> KSYIDRDTEYLLQENEPNLSLDQHLLEDLQRKKTDPRYIEMQRFRKKLPSYGMQKELVNLINNHQVTVISGETGCGKTTQVTQFILDNYIERGKGSACRIVCTQPRRISAISVAERVATERAESCGNGNSTGYQIRLQSRLPRKQGSILYCTTGIILQWLQSDSRLSSVSHIVLDEIHERNLQSDVLMTVIKDLLHFRSDLKVILMSATLNAEKFSEYFGNCPMIHIPGFTFPVVEYLLEDIIEKIRYVPDQKEHRSQFKRGFMQGHVNRQEKEEKEAIYKERWPAYIKELRTRYSASTVDVLQMMDDDKVDLNLIAALIRYIVLEEEDGAILVFLPGWDNISTLHDLLMSQVMFKSDKFLIIPLHSLMPTVNQTQVFKKTPPGVRKIVIATNIAETSITIDDVVYVIDGGKIKETHFDTQNNISTMSAEWVSKANAKQRKGRAGRVQPGHCYHLYNGLRASLLDDYQLPEILRTPLEELCLQIKILRLGGIAYFLSRLMDPPSNEAVVLSIKHLMELSALDKQEELTPLGVHLARLPVEPHIGKMILFGALFCCLDPVLTIAASLSFKDPFVIPLGKEKIADARRKELAKETRSDHLTVVNAFEGWEEAKRRGFRYEKDYCWEYFLSSNTLQMLHNMKGQFAEHLLGA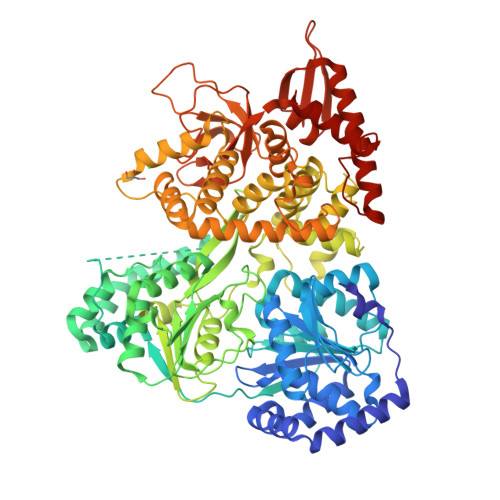GFVSSRSPKDPKANINSDNEKIIKAVICAGLYPKVAKIRLNLGKKRKMVKVHTKSDGLVSIHPKSVNVEQTDFHYNWLIYHLKMRTSSIYLYDCTEVSPYCLLFFGGDISIQKDKDQEIIAVDEWIVFQSPERIAHLVKGLRKELDSLLQEKIESPHPVDWDDTKSRDCAVLSAILDLIKT>[2x]GGGAGCCCUGUCACCGGAUGUGCUUUCCGGUCUGAUGAGUCCGUGAGGACAAAACAGGGCUCCCGAAUU

The hammerhead ribozyme, since its discovery in satellite virus RNA genomes, has been a central focus of experiments designed to correlate RNA structure with RNA catalysis, as it is a comparatively small RNA whose biochemistry has been intensively investigated using a wide variety of approaches. The most well-characterized member of the first class of natural hammerheads occurs within the satellite RNA of the tobacco ringspot virus (sTRSV), which is also the first hammerhead ribozyme discovered. Instead of inactivating the nucleophile via methylation, as was done with the Schistosome hammerhead, the cleavage reaction in the case of the sTRSV hammerhead has been greatly decelerated with a G12A enzyme active site variant that lowers the pKa of the purine general base in the cleavage reaction from approximately 9.5 to approximately 3.5, which, assuming the observed log-linear rate dependence on pH, potentially represents an approximately 106-fold decrease of the reaction rate. By greatly slowing the reaction, the hammerhead RNA crystallizes prior to cleavage, but remains active in the crystal and slowly cleaves.

Two precatalytic (uncleaved) models were unambiguously constructed in the 2.4 Å electron density map and refined. The precleavage or enzyme–substrate complex structure of the G12A sTRSV hammerhead RNA at 2.4 Å resolution reveals an active site very similar to that of the Smα hammerhead, despite the presence of the 2′-OMe modification in the latter, and the G12A substitution in sTRSV hammerhead. Hence, it is reasonable to conclude that neither modification grossly perturbs the atomic structure of the hammerhead ribozyme active site. Some small differences between the sTRSV hammerhead enzyme–substrate complex structure and the corresponding Smα hammerhead enzyme–inhibitor complex do exist. The unmodified 2′-OH of C17 in the latter appears to be slightly more in-line with the scissile phosphate (168.5° vs. 162°), and the position of A12 differs slightly, due to a different hydrogen-bonding interaction with A9 that replaces the G12/A9 sheared pairing. The geometry of the G12A sTRSV appears to be somewhat better suited to initiation of the cleavage reaction. Specifically, the angle between the N1 of A12, the 2′O nucleophile (C17), and the adjacent scissile phosphorus is 149°, and the distance between N1 and O2′ is 2.7 Å. The in-line attack angle (between O2′, P, and O5′) is 168° in the G12A structure, versus 162° in the previous G12 structure. Hence, the slow cleavage rate appears to be primarily due to the result of the purine pKa shift from approximately 9.5 to approximately 3.5 upon G12A substitution, rather than due to a disadvantageous structural perturbation. In this sense, A12 may be a better (albeit much slower) representation of the activated ribozyme poised for general base catalysis, even though A12 is a much weaker base than G12 due to its much smaller pKa.> MVKRFSTAYLLLGIL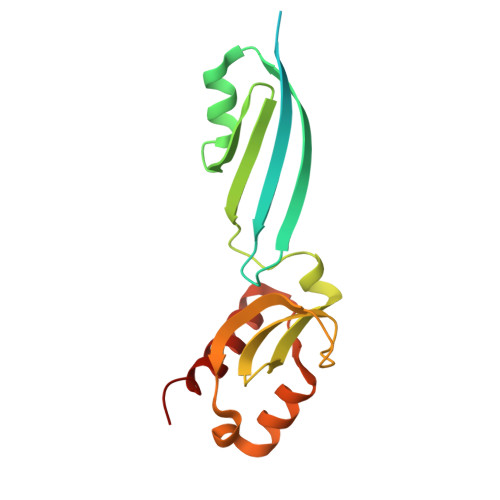CSAAVFLIGAPSRALGAEVEHYEPLQVHVQLEKVYLDGDVSIEHKHEKVFSMDDFWAAYAGWTLVEQKKGYVLFRKQMDDISPLSKVNGYIGVSDNGVISTFHGRPEPASEPIQSFFQIDLERLESHMQKNLLKGIPFRTKAEFEDVIEHMKTYSGLE> VQTVPLSRLFDH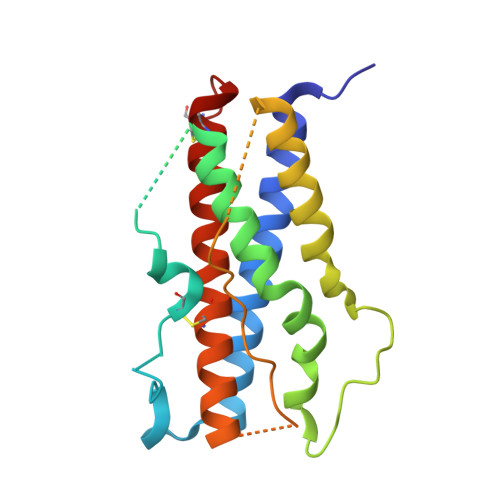AMLQAHRAHQLAIDTYQEFEETYIPKDQKYSFLHDSQTSFCFSDSIPTPSNMEETQQKSNLELLRISLLLIESWLEPVRFLRSMFANNLVYDTSDSDDYHLLKDLEEGIQTLMGRLEDGSRRTGQILKQTYSKFDTNSHNHDALLKNYGLLYCFRKDMDKVETFLRMVQCRSVEGSCGF> ANELTWHDVLAEEKQQPYFLNTLQTVASERQSGVTIYPPQKDV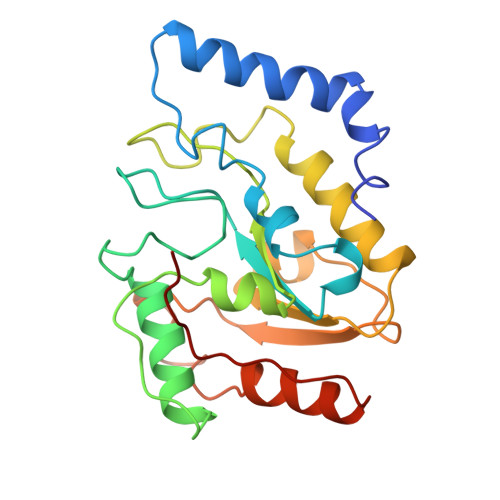FNAFRFTELGDVKVVILGQDPYHGPGQAHGLAFSVRPGIAIPPSLLNMYKELENTIPGFTRPNHGYLESWARQGVLLLNTVLTVRAGQAHSHASLGWETFTDKVISLINQHREGVVFLLWGSHAQKKGAIIDKQRHHVLKAPHPSPLSAHRGFFGCNHFVLANQWLEQRGETPIDWMPVLPAESE>GGELMIKSSNAFDVIELSS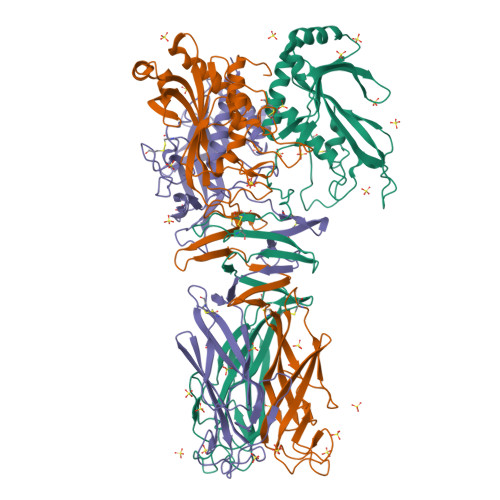QIQRYASLSKINNRTNPILKDNKAKEFKDADLKWLKLENCPTAGDVPTTGNNNDLQDQFIACDADYRKGDLSYFGSQFEFSTYVHPSNPEIQRQIKQVVSYFQYRGMERAFIGDAAGYVISEAKKKGFSAQDYRIVLIEPDRVGYFESNAISYEEFIENPSARENFLLKATKDRTLALAVSLAQTGEIAMQRDGSVAFLEDSELCWDTAAGSAKSCLSVRYDTVGNKTELDLKQIDVVSAKGLSFESDGKTKTPVVSTYETFQDGGRAKTINAIECPTGLNNRFAAVVSSFSTAGQNANFSSESAKDSQGTTQKDGSKGPHALLSGISLNWTLTNKVWDVTASIGIESGILPTSGIDSGSLLRNPKSLSFIAFQWCEN[3x]>[2x]GPDSMSTSSHTVLLIQTSPRLDSRTWGDYESVTDALDALCKMFEDFLS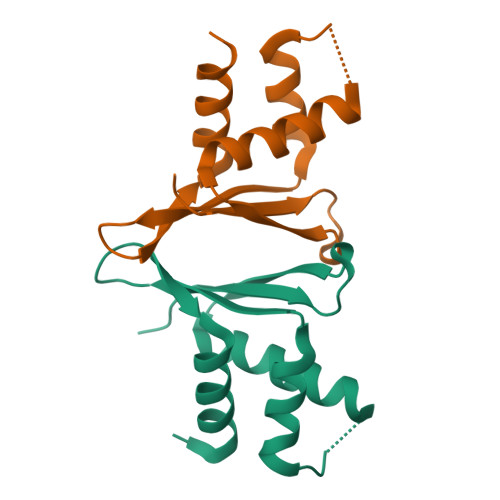KKSAAPVTYDVSQVYEFLDKLSDVSMMIFNRETGQYIGRTRAWIKQQVYEMMRGR>MSLENIMTLPKIKHVRAWFIGGATAEKGAGGGDYHDQGGNHWIDDHIATPMSKYRDYEQSRQSFGINVLGTLIVEVEAENRQTGFAVSTAGEMGCFIVEKHLNRFIEGKCVSDIKLIHDQMLGATMYYSGSGGLVMNTISCVDLALWDLFGKVVGLPVYKLLGGAVRDEIQFYATGARPDLAKEMGFIGGKMPTHWGPHDGDAGIRKDAAMVADMREKCGPDFWLMLDCWMSQDVNYATKLAHACAPFNLKWIEECLPPQQYEGYRELKRNAPAGMMVTSGEHHGTLQSFRTLAETGI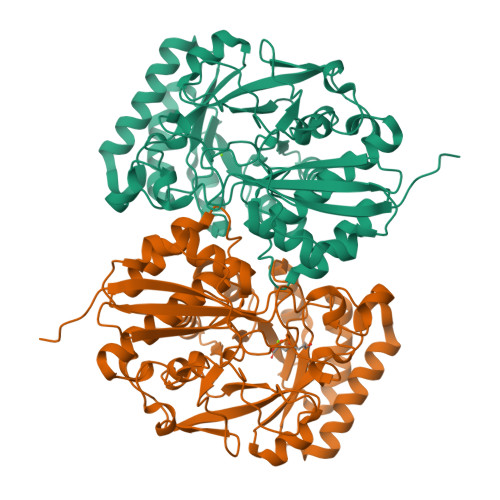DIMQPDVGWCGGLTTLVEIAALAKSRGQLVVPHGSSVYSHHAVITFTNTPFSEFLMTSPDCSTLRPQFDPILLDEPVPVNGRIHKSVLDKPGFGVELNRDCHLKRPYSHEGHHHHHH[2x]As the most abundant viral protein encoded by the M gene segment, matrix protein 1 (M1) forms a shell underneath a host cell-derived lipid biolayer to connect the vRNPs with the viral envelope in mature virions. The full-length M1 protein includes 252 amino acids consisting of a highly organized N-terminal domain and a flexible but less ordered C-terminal domain that are linked by a protease-sensitive loop. So far, only the N-terminal domain of M1 has been structurally resolved at an atomic level, showing that at neutral pH the physiological monomers have a high tendency to oligomerize via a so-called ‘face-to-back’ arrangement, whereas at acidic pH the N-terminal domain exists as a dimeric structure in a so-called ‘face-to-face’ arrangement.

G88R but not G88E was originally acquired by the virus as a spontaneous compensatory mutation after NLS disruption. M(NLS-88R) M1, similar to wt-M1, is able to switch from a face-to-back monomer–monomer association at neutral pH to a face-to-face-oriented dimeric conformation at acidic pH. The residues Lys104 (part of the NLS motif), Arg134, Tyr100 and Asp94 on the ‘face’ of one molecule (Monomer A) interact with several complementary residues on the ‘back’ of a second molecule (Monomer B), including Glu29, Asp30, Lys21 and Ser17. The face-to-back monomeric arrangement of M1 occurring at neutral pH is likely necessary for the formation and maintenance of a confluent and strong matrix layer underneath the viral envelope, whereas the face-to-face dimeric arrangement at acidic pH may describe M1 that has dissociated from the extended matrix layer. We then determined M1–M1 interactions under different pH conditions by BLI. Regardless of pH conditions, M(NLS-88R) had M1–M1 interactions in a dose-dependent manner similar to wt-M1 (Figure 3A vs 3B and Figure 3D vs 3E). Nevertheless, M(NLS-88R) M1 retains pH-dependent conformational transition like WSN. Compared with M(NLS-88E), that M(NLS-88R) has less difficulty to break the fulcrum likely translates into a smaller cooperative energy requirement of monomer-to-dimer conversion under subtle pH changes. This flexibility facilitates M(NLS-88R) M1 to dissociate from vRNP in the acidified endosome, thus prompting virus replication in vitro. Our results also indicate that the compensatory G88R mutation was not a random mutation but was chosen by the virus purposefully to retain pH-dependent conformational flexibility for efficient virus replication.

> MHHHHHHSLLTEVETYVLSIVPSGPLKAEIAQRLEDVFAGKNTDLEVLMEWLKTRPILSPLTKGILGFVFTLTVPSERGLQRRRFVQNALNGNRDPNNMDKAVKLYSKLKSEITFHGAKEIALSYSAGALASCMGLIYNRMGAVTTEVAFGLVCATCEQIADSQHRSHRQM>HHHHHHENLYFQGMSFDNYLVPTVIEQSGRGERAFDIYSRLLKERIVFLVGPVTDESANLVVAQLLFLESANPDKDIFFYINSPGGSVTAGMSIYDTMNFIKPDVSTLCLGQAASMGAFLLSAGEKGKR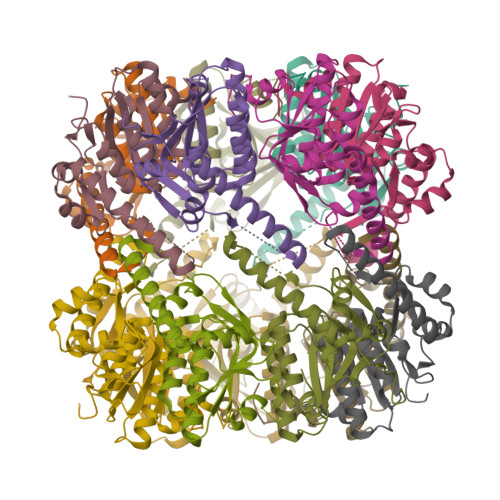FALPNSRIMIHQPLISGGLGGQASDIEIHARELLKIKEKLNRLMAKHCDRDLADLERDTDRDNFMSAEEAKEYGLIDQILENRASLRL[14x]>HHHHHHSSGLVPRGSHMRVLALSAVFLVASIIGMPAVAKEWQENKSWNAHFTEHKSQGVVVLWNENKQQGFTNNLKRANQAFLPASTFXIPNSLIALDLGVVKDEHQVFKWDGQTRDIATWNRDHNLITAMKYSVVPVYQEFARQIGEARMSKMLHAFDYGNEDISGNVDSFWLDGGIRISATEQISFLRKLYHNKLHVSERSQRIVKQAMLTEANGDYIIRAKTGY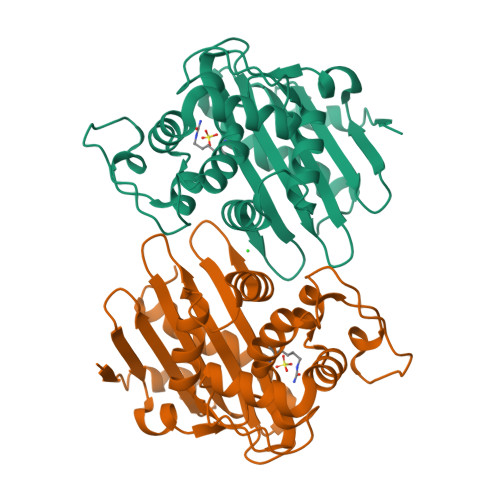STRIEPKIGWWVGWVELDDNVWFFAMNMDMPTSDGLGLRQAITKEVLKQEKIIP[2x]 3',4'-demethoxy-nogalose-1-hydroxy-nogalamycinone | C29 H32 O13 | 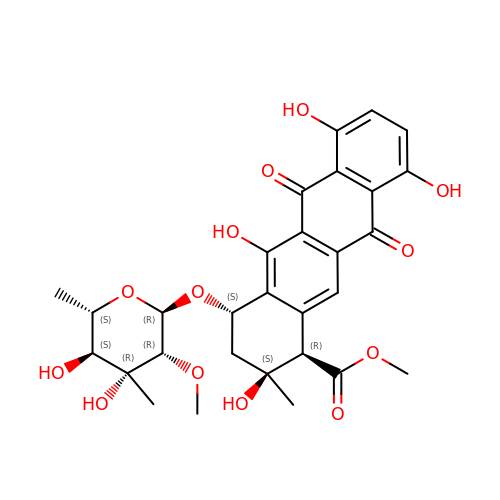JMZPXXMAMHNKHM-WOAFMFBISA-N> ATTLYLTRHGETKWNVERRMQGWQDSPLTEKGR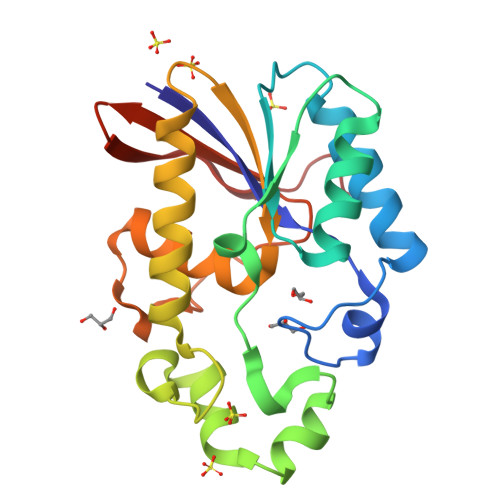QDAMRLGKRLEAVELAAIYTSTSGRALETAEIVRGGRLIPIYQDERLREIHLGDWEGKTHDEIRQMDPIAFDHFWQAPHLYAPQRGERFCDVQQRALEAVQSIVDRHEGETVLIVTHGVVLKTLMAAFKDTPLDHLWSPPYMYGTSVTIIEVDGGTFHVAVEGDVSHIE> MTQVASPVVQARYSPVELSAALGLFPPTDEQAAVIAAPPGPLVVIAGAGAGKTETMAARVVWLVANGFATPSQVLGLTFTRKAAGQLLRRVRTRLARLAGAGLAPGSGASDESATVSTYHAFAGTLLREHGLLLPVEPDTRLLSETELWQLAYDVVCAHPGHLDTEKTPAAVTAMVLRLSGALAEHLVDTDQLRDTHVELERLVHTLPAGPYQRDRGPSQWLLRMLATQTERTELVPLIDALHQRMRAEKVMDFGMQMAAAARLAARFPQVGEQLRQRFRVVLLDEYQDTGHAQRIALSSLFGGGADDGLALTAVGDP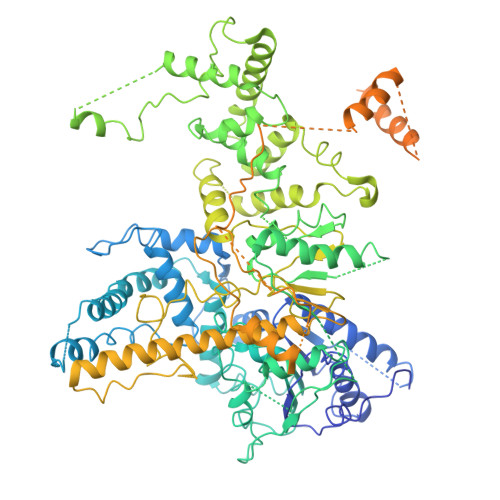IQSIYGWRGASATNLPRFTTDFPYSDGTPAPTLELRTSWRNPPSTLHVANAVSEEARRRSVAVRALRPRPDAEPGTIRCALLNNVAAERDWVADHLARAYHGAIGRGEAAPTAAVLVRRNADAAPMAEALTARGVPVEVVGVAGLLAVPEVADLVAMLRLIADPTAGSAVMRILTGPRWRFGARDIAALWRRAVELDDRPKGELGTADIVAQAAPDADTACVADAICDPGDAERYSPAGYERIVALGRELTMLRAHLGHPLPELVAEVRRVLGLDAEARAARPVAAGWAGTENLDRFSDLVSDFAGHAGASVSALLAYLDAAVEVENGLAPAELTVSHDRVQILTVHAAKGLEWQVVAVPHLSARVFPSTTQARTWLTDASDLPPLLRGDRATESEIGVPVLDTSDIYDRKILSDKISDHKKSLDQRRVDEERRLLYVAITRAEDTLLLSGHHWGATESKPRGPSEFLCELKTILEEATAAGTPCGEIEHWAPDPAPGETNPLRDQVVEALWPPVASADDHVHRGAQLVAAAMAGEVSAEADQEGWAADVDALLAERERPPQQEDTELPGQLSVSTLVELSRDPKAALTRLRRRLPQRPDPHALLGTTFHEWVQRYFHAERLFDLDDLPGAVDSDSGRAVEESLAELQDAFVKSPWAARTPVEVEVPFDMVLGETVVRGRIDAVFAEPDGTTMVLAWKTGDPPETPEAKEHAAVQLAVYRLAWAAMRGCPPESVRAAFHYVRSGQTVIPETLPGAEELVKLLAAAPTETAEEADRIT(4S)-4-methyl-1,4,5,6-tetrahydropyridin-2-amine | C6 H12 N2 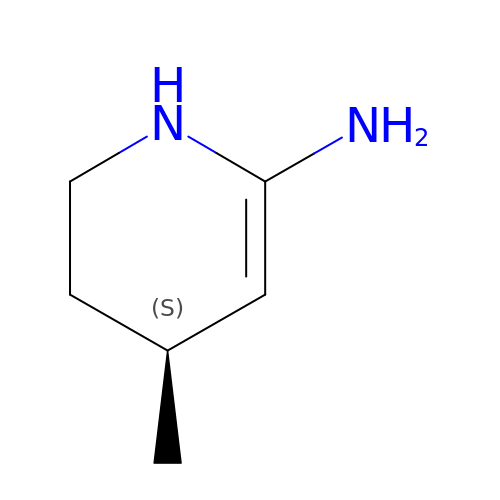| XSGKRRZSNPERQU-YFKPBYRVSA-N>ASMTGGQQMGRDEAGITGTWYNQLGSTFIVTAGADGALTGTYESAVGNAESRYVLTGRYDSAPATDGSGTALGWTVAWKNNYRNAHSATTWSGQYVGGAEARINTQWLLTEGTTEANAWHSTLVGHDTFTKVKPSAASIDAA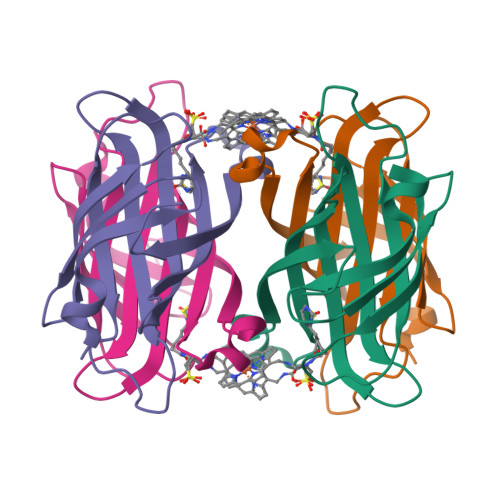KKAGVNNGNPLDAVQQ[4x]> GSTREPEIASSLIKQIFSHYVKTPVTRDAYKIVEKCSERYFKQISSDLEAYSQHAGRKTVEMADVELLMRRQGLVTDKMPLHVLVERHLPLE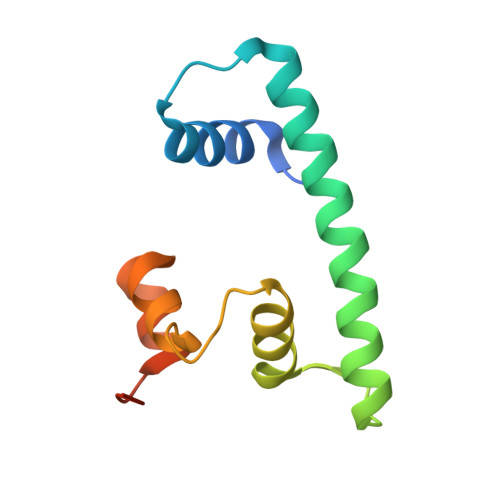YRKLLIPIAVSGNKVIPCK AtBFN2 (also called ENDO2) is a 34.5 kDa glycoprotein (the predicted mass for protein component alone is 30.5 kDa), encoded by the Arabidopsis thaliana At1g68290 gene. AtBFN2 follows the standard glycosylation pattern of plant S1/P1 endonucleases, with three glycosylation sites (Asn91, Asn110, and Asn184). While the P1 nuclease has a higher specificity for RNA over ssDNA, in a previous study we showed that the opposite is true for AtBFN2. Structurally, Zn2+-dependent endonucleases present a unique fold, and are classified into the P1/S1 nuclease family (pfam ID PF02265), itself part of the Phospholipase C (PLC)/P1 nuclease superfamily (pfam ID CL0368).

We obtained a ligand-free AtBFN2 structure, as well as a phosphate co-crystal structure in a new unit cell with space group P1. In addition to our improved AtBFN2•SO4 co-crystal structure, we were also able to obtain a new, ligand-free, structure, which was solved from crystals belonging to space-group P 1. In this structure, we found that four water molecules coordinate the tri-metallic cluster. Finally, water four (Wat4) coordinates Zn1. Wat1 is in the predicted required position for an activated nucleophile, further strengthening our earlier proposal for a reaction mechanism.

>WGKEGHEIICKIAQTRLDETAAKAVKELLPESAEGDLSSLCLWADRVKFRYHWSSPLHYINTPDACSYQYNRDCKDESGEKGRCVAGAIYNYTTQLLSYKTAASSQSQYNLTEALLFVSHFMGDIHQPLHVSYASDKGGNTIEVHWYTRKANLHHIWDSNIIETAEADLYNSALEGMVDALKKNITTEWADQVKRWETCTKKTACPDIYASEGIQAACDWAYKGVTEGDTLEDEYFYSRLPIVYQRLAQGGVRLAATLNRIFGHHHHHH[2x]>MTTAAGLSGIDLTDLDNFADGFPHHLFAIHRREAPVYWHRPTEHTPDGEGFWSVATYAETLEVLRDPVTYSSVTGGQRRFGGTVLQDLPVAGQVLNMMDDPRHTRIRRLVSSGLTPRMIRRVEDDLRRRARGLLDGVEPGAPFDFVVEIAAELPMQMICILLGVPETDRHWLFEAVEPGFDFRGSRRATMPRLNVEDAGSRLYTYALELIAGKRAEPADDMLSVVANATIDDPDAPALSDAELYLFFHLLFSAGAETTRNSIAGGLLALAENPDQLQTLRSDFELLPTAIEEIVRWTSPSPSKRRTASRAVSLGGQ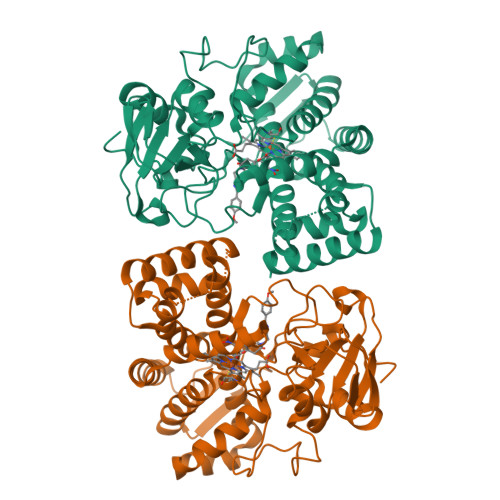PIEAGQKVVVWEGSANRDPSVFDRADEFDITRKPNPHLGFGQGVHYCLGANLARLELRVLFEELLSRFGSVRVVEPAEWTRSNRHTGIRHLVVELRGG[2x]>[2x]ATQTVTLSVPGMTCSACPITVKKAISKV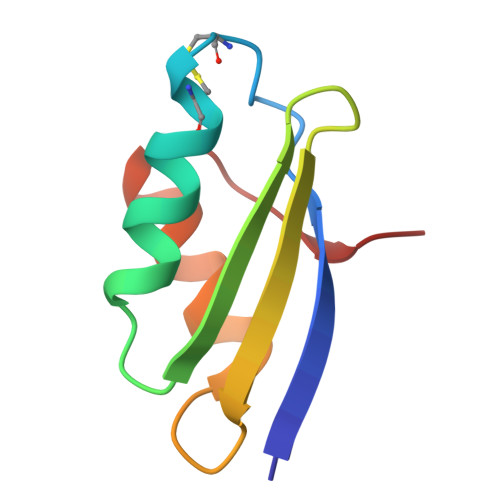EGVSKVDVTFETRQAVVTFDDAKTSVQKLTKATADAGYPSSVKQ(3S)-piperidin-3-ol 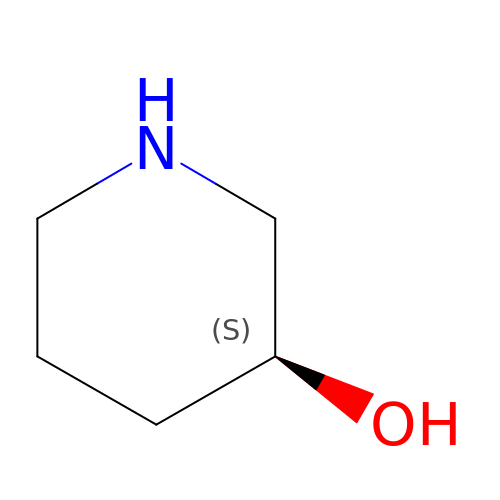| C5 H11 N O | BIWOSRSKDCZIFM-YFKPBYRVSA-N>[6x]MTLYRLHEADLEIPDAWQDQSINIFKLPASGPAREASFVISRDASQGDAPFADYVARQLENAEKQLPGFKLHKRWDINIHGHAAVLLDYQWQREGRDLMLRQVFIERRPAVLITTLTTTPADLPHHEPAWKQAMQTLVPRPTPSGS;>[3x]MDAQAAARLGDEIAHGFGVAAMVAGAVAGALIGAAVVAATAATGGLAAVILAGSIAAGGLSHHHHHH

One such pathway is the type VI secretion system (T6SS), which in many bacterial species functions to deliver antibacterial effector proteins from the cytoplasm directly into an adjacent bacterial cell via a one-step secretion event. In contrast, DUF1795 proteins, also known as effector-associated gene (Eag) chaperones, interact with so-called ‘evolved’ PAAR proteins in which the PAAR and toxin domains are found as a single polypeptide chain. Crystal structures of Eag chaperones in complex with the TMDs of cognate class I and class II effectors reveal the conformation of effector TMDs prior to their secretion and insertion into target cell membranes. Given that the Eag chaperone dimer creates a hydrophobic environment with complementary knob-hole interactions for its cognate effector TM helices, and interacts with TM helices via side chain to main chain hydrogen bonds, we conclude that Eag chaperones provide an environment that mimics transmembrane helical packing to stabilize prePAAR effector TMDs in the cytoplasm prior to effector export from the cell.

The structure of the EagT6 chaperone was previously solved as part of a structural genomics effort and we were additionally able to obtain a 2.60 Å co-crystal structure of this chaperone in complex with the N-terminal prePAAR and first TMD region of the class II effector Tse6 (Tse6NT). A comparison of the chaperone structures in their apo and effector-bound states shows that upon effector binding, both chaperones ‘grip’ the prePAAR-TMD region of their cognate effector in a claw-like manner. By contrast, Tse6NT exhibits a pseudosymmetric binding mode with EagT6. In this structure, two alpha-helices of Tse6 each occupy equivalent Eag binding pockets and run in the opposite direction to match the antiparallel arrangement of the EagT6 dimer. For example, A7 and A30 of Tse6 interact with equivalent sites in their respective chaperone protomers. These two helices, which consist of prePAAR and a TM helix, flank a central TM helix whose C-terminus extends into the solvent, likely indicating the location of the downstream PAAR domain in the full-length effector. By contrast, we were able to model the entire prePAAR motif of Tse6NT and in this case, the motif forms an alpha helix that binds the hydrophobic pocket of an EagT6 protomer. In this structure, the two conserved alanine residues of prePAAR make contact with the EagT6 chaperone, whereas the arginine, aspartate and histidine residues are solvent exposed. It should be noted that the modelled conformation of Tse6NT appears to be locked into place by crystal packing, suggesting that in solution Tse6’s prePAAR motif may exhibit significant conformational flexibility and can dissociate from EagT6 as is observed for the prePAAR motif of Rhs1. For example, I22 and I24 of EagT6 create a hydrophobic surface in the ‘palm’ of the claw, which is flanked on either side by symmetrical hydrophobic surfaces comprised of A62, L66, L98, F104, and I113.>XGELEALAQELEALAKKLKALAW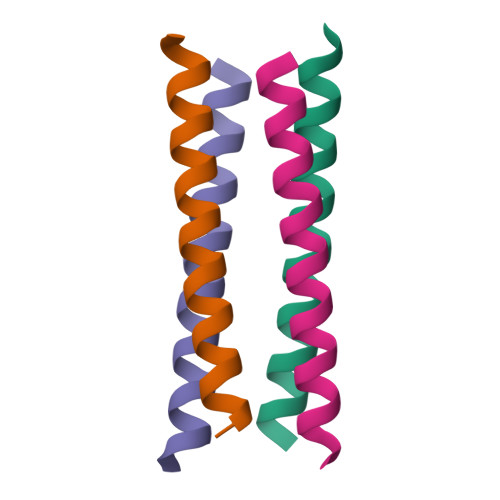KLKALAQGX[4x]>MAHHHHHHMSLAVEAVKDFLLKLQDDICEALEAEDGQATFVEDKWTREGGGGGRTRVMVDGAVIEKGGVNFSHVYGKGLPMSSTERHPDIAGCNFEAMGVSLVIHPKNPHVPTSHANVRLFVAEREGKEPVWWFGGGFDLTPYYAVEEDCRDFHQVAQDLCKPFGADVYARFKGWCD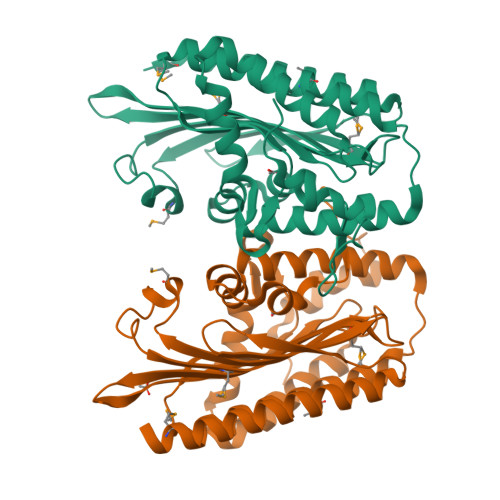EYFFIPYRNEARGIGGLFFDDLNEWPFEKCFEFVQAVGKGYMDAYIPIVNRRKNTPYTEQQVEFQEFRRGRYAEFNLVIDRGTKFGLQSGGRTESILISLPPRARWGYNWQPEPGTPEARLTEYFLTKRQWV[2x]>[2x]MAKG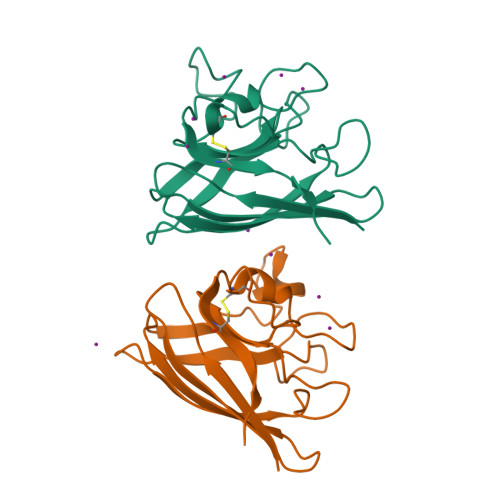VAVLSSSEGVAGTILFTQEGDGPTTVTGNISGLKPGLHGFHVHALGDTTNGCMSTGPHFNPAGKEHGSPEDETRHAGDLGNITVGDDGTACFTIVDKQIPLTGPHSIIGRAVVVHADPDDLGKGGHELSKSTGNAGGRIACGIIGLQG>[8x]MSLTSEDFLIKSKGYLDIQTGEIIKADLLIRNGKIAEIGKINTKDATVISIPDLILIPGLMDSHVHIVGNDSKGEESIADSSHMGTVWGVVNAEKTLMAGFTTVRNVGAANYADVSVRDAIERGVINGPTMLVSG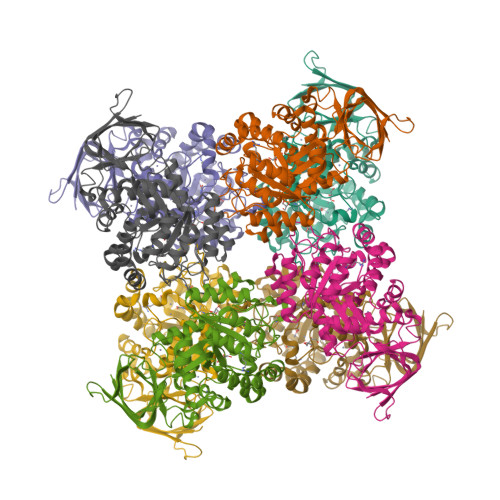PALGITGGHCDHNLLPPEFNYSSEGVVDSPWEARKMVRKNRKYGADLIKFCATGGVMSRNTDVNAKQFTLEEMKAIVDEAHNHGMKVAAHAHGLIGIKAAIKAGVDSVEHASFIDDETIDMAIKNNTVLSMDIFVSDYILGEGAKAGIREESLNKERLVGKKQRENFMNAHRRGAIITFGTDAGIFDHGDNAKQFAYMVEWGMTPLEAIQASTIKTATLFGIENIGQIKEGFDADIVGVIENPLANIRTLEEVAFVMKEGKVYKREGHHHHHH>[16x]SNAMAEDKGRKVVVSALQFACTDDVSTNVTTAERLVRAAHKQGANIVLIQELFEGYYFCQAQREDFIQRAKPYKDHPTIMRLQKLAKELGVVIPVSFFEEANNAHYNSIAIIDADGTDLGIYRKSHIPDGPGYEEKFYFNPGDTGFKVFQTKYAKIGVAICWDQWFPEAARAMALQGAEILFYPTAIGSEPHDQSIDSRDHWKRVMQGHAGANLVPLVASNRIGNEIIETEHGKSEIKFYGNSFIAGPTGEIVSIADDKEEAVLIAEFNLDKIKSMRHCWGVFRDRRPDLYKVLLTLDGKNPVL

The arginine route involves three enzymatic steps: (i) arginine decarboxylation to agmatine by arginine decarboxylase (ADC, EC 4.1.1.19); (ii) deimination of agmatine by agmatine iminohydrolase (AIH, EC 3.5.3.12) and (iii) hydrolysis of N-carbamoylputrescine (NCP) to putrescine by N-carbamoylputrescine amidohydrolase (CPA, EC 3.5.1.53), with the release of carbon dioxide and ammonia. N-carbamoylputrescine amidohydrolase enzymes belong to nitrilases, and more precisely, to C-N hydrolases breaking non-peptide bonds using Cys-Glu-Lys catalytic triad. The octameric MtCPA enzyme is assembled into an incomplete helical twist, made by four tight dimers with swapped C-termini. As in other nitrilases, the substrate hydrolysis is carried out by the catalytic triad, composed in MtCPA of Glu48 (proton acceptor), Lys121 (proton donor) and Cys158 (nucleophile).

The structures of wild-type MtCPA, crystallized in the presence of PUT and CAD in the solution, were determined at 1.97 and 2.19 Å resolution, respectively. In that instance, there would be not enough room to bind entire CAD molecule. This is not the case, and we do indeed observe CAD in the active site. CAD in MtCPA complex reaches deeper than PUT into the catalytic pocket, however, due to presence of sulfhydryl group of Cys158 it bends toward Glu132. All bound amines, CAD, PUT and DHMP, present the same hydrogen bond between terminal amine group and the side chain oxygen of Glu187. Although CAD is able to interact via hydrogen bond with Glu187 at the entrance of the pocket, similarly to PUT and DHMP, deep inside the cleft CAD passes by the Sγ of Cys158 and bends toward the pair of glutamates. Thus, this would not leave enough space for the carbamoyl moiety of such longer substrate. From the MtCPA/CAD complex, we can assume that longer substrates than NCP, such as N-carbamoylcadaverine, would not obtain stable conformation inside the active site. In other words, the proper orientation of N-carbamoylcadaverine, with the preservation of the hydrogen bond with the Glu187 side chain is impossible due to steric clashes either with the catalytic triad or with the residues in the middle section of the pocket.> MAWPKVQPEVNIGVVGHVDHGKTTLVQAITGIWTSKKLGYAETNIGVCESCKKPEAYVTEPSCKSCGSDDEPKFLRRISFID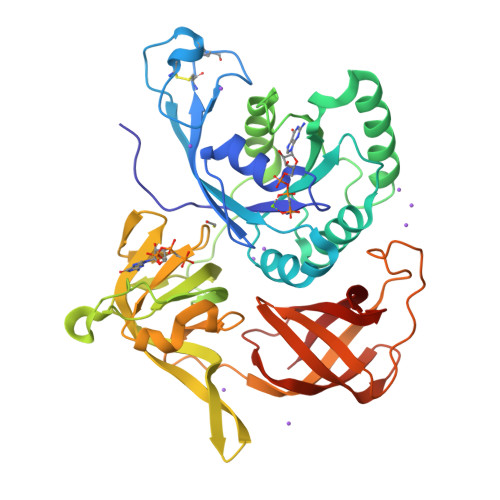APGHEVLMATMLSGAALMDGAILVVAANEPFPQPQTREHFVALGIIGVKNLIIVQNKVDVVSKEEALSQYRQIKQFTKGTWAENVPIIPVSALHKINIDSLIEGIEEYIKTPYRDLSQKPVMLVIRSFDVNKPGTQFNELKGGVIGGSIIQGLFKVDQEIKVLPGLRVEKQGKVSYEPIFTKISSIRFGDEEFKEAKPGGLVAIGTYLDPSLTKADNLLGSIITLADAEVPVLWNIRIKYNLLERVVGAKEMLKVDPIRAKETLMLSVGSSTTLGIVTSVKKDEIEVELRRPVAVWSNNIRTVISRQIAGRWRMIGWGLVEI>[2x]GSTANESALQTLLADMRGKIGEIVGIAGNSDQNLTKVKLQYQKAHNELNETHQFFASMLDERKTELLKELETLYTAKVNSNNSWQQRSRDLIDKGLATCEAVERSPAPPSSLLTEALLLRKS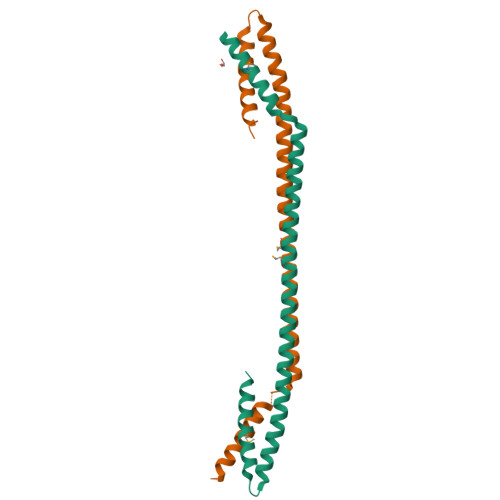LEQQLQTGIQEMQL> GSHMEEIRNLTVKDFRVQELPLARIKKIMKLDEDVKMISAEAP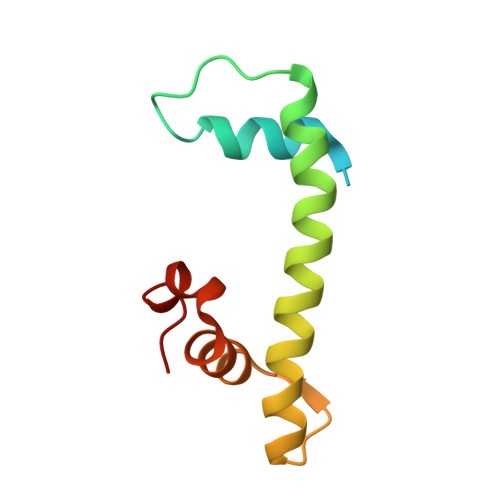VLFAKAAQIFITELTLRAWIHTEDNKRRTLQRNDIAMAITKFDQFDFLIDIVPR> MINMTRK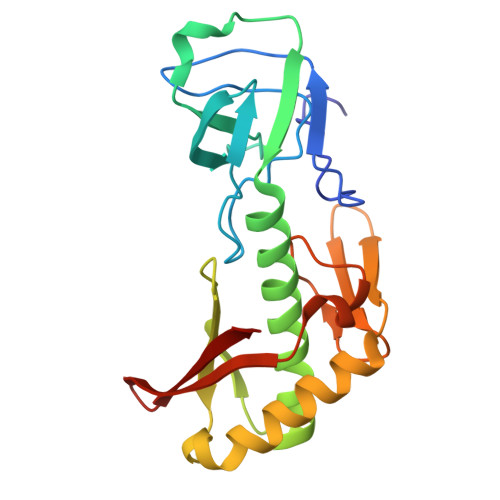LYYEDAYLKEAKGRVLEIRDNAILLDQTIFYPTGGGQPHDRGTINGVEVLDVYKDEEGNVWHVVKEPEKFKVGDEVELKIDWDYRYKLMRIHTGLHLLEHVLNEVLGEGNWQLVGSGMSVEKGRYDIAYPENLNKYKEQIISLFNKYVDEGGEVKIWWEGDRRYTQIRDFEVIPCGGTHVKDIKEIGHIKKLKRSSIGRGKQRLEMWLE>GAMDTPGPPQDLKVKEVTKTSVTLTWDPPLLDGGSKIKNYIVEKRE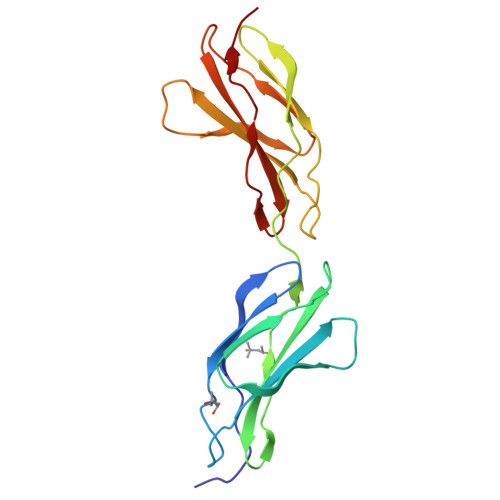STRKAYSTVATNCHKTSWKVDQLQEGCSYYFRVLAENEYGIGLPAETAESVKASERPLPPGKITLMDVTRNSVSLSWEKPEHDGGSRILGYIVEMQTKGSDKWATCATVKVTEATITGLIQGEEYSFRVSAQNEKGISDPRQLSVPVIAKD[2x]>NLYQFKNMIQCTVPSRSWWDFADYGCYCGRGGSGTPVDDLDRCCQVHDNCYNEAEKISGCWPYFKTYSYECSQGTLTCKGGNNACAAAVCDCDRLAAICFAGAPYNDNDYNINLKAR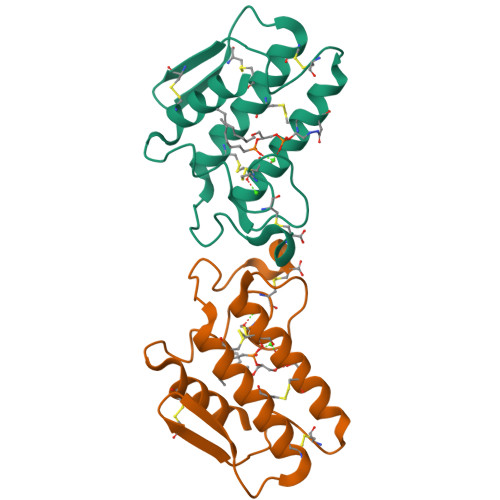C[2x]> MFHSSAMVNSHRKPMFNIHRGFYCLTAILPQICICSQFSVPSSYHFTEDPGAFPVATNGERFPWQELRLPSVVIPLHYDLFVHPNLTSLDFVASEKIEVLVSNATQFIILHSKDLEITNATLQSEEDSRYMKPGKELKVLSYPAHEQIALLVPEKLTPHLKYYVAMDFQAKLGDGFEGFYKSTYRTLGGETRILAVTDFEPTQARMAFPCFDEPLFKANFSIKIRRESRHIALSNMPKVKT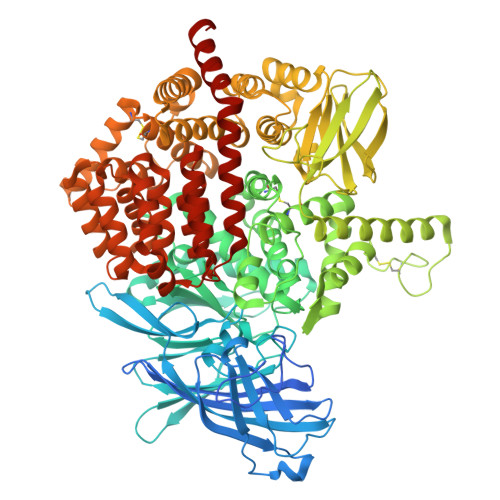IELEGGLLEDHFETTVKMSTYLVAYIVCDFHSLSGFTSSGVKVSIYASPDKRNQTHYALQASLKLLDFYEKYFDIYYPLSKLDLIAIPDFAPGAMENWGLITYRETSLLFDPKTSSASDKLWVTRVIAHELAHQWFGNLVTMEWWNDIWLNEGFAKYMELIAVNATYPELQFDDYFLNVCFEVITKDSLNSSRPISKPAETPTQIQEMFDEVSYNKGACILNMLKDFLGEEKFQKGIIQYLKKFSYRNAKNDDLWSSLSNSCLESDFTSGGVCHSDPKMTSNMLAFLGENAEVKEMMTTWTLQKGIPLLVVKQDGCSLRLQQERFLQGVFQEDPEWRALQERYLWHIPLTYSTSSSNVIHRHILKSKTDTLDLPEKTSWVKFNVDSNGYYIVHYEGHGWDQLITQLNQNHTLLRPKDRVGLIHDVFQLVGAGRLTLDKALDMTYYLQHETSSPALLEGLSYLESFYHMMDRRNISDISENLKRYLLQYFKPVIDRQSWSDKGSVWDRMLRSALLKLACDLNHAPCIQKAAELFSQWMESSGKLNIPTDVLKIVYSVGAQTTAGWNYLLEQYELSMSSAEQNKILYALSTSKHQEKLLKLIELGMEGKVIKTQNLAALLHAIARRPKGQQLAWDFVRENWTHLLKKFDLGSYDIRMIISGTTAHFSSKDKLQEVKLFFESLEAQGSHLDIFQTVLETITKNIKWLEKNLPTLRTWLMVNTRHHHHHH MaeK and MaeR exert their function by activating the expression of L-malate catabolic genes (maeP and maeE) and the expression of their own genes upon the presence of L-malate in the medium. Structural and phylogenetic analyses show that L. casei MaeKR proteins belong to the citrate family of TCS, as well as the characterized DcuSR and CitAB TCS. We also solved the crystal structure of the REC domain of MaeR in its activated state as well as the structure of a mutant version defective in the phosphoacceptor Asp. Altogether, our analysis has revealed that MaeKR is a non-canonical TCS conserved in Lactobacillales and that the structure of MaeR acknowledges the α4β5α5-swapped dimers as a new class of dimerization for RRs.

In an attempt to determine the MaeR unphosphorylated monomeric conformation, we performed crystallization studies of a MaeRREC mutant form where D54 was replaced by an alanine (MaeRREC-D54A). MaeRREC-D54A crystallized in the same space group and similar size dimension than the wild-type MaeRREC. The determination of the structure of MaeRREC-D54A by molecular replacement revealed the presence of a swapped dimer into the unit cell identical to the one obtained for the wild type MaeRREC (RMSD is 0.52 Å for 242 residues). The crystals were obtained at high concentrations of sulfate (1.6 M) and it is well known that sulphates can mimic phosphate ions. No interactions with the conserved Asp9 were observed due to the absence of a magnesium ion in the active site. The residues Thr82 and Tyr101 forming the Y-T switch present the inward conformation as in the MaeRREC-BeF structure, confirming an activated state for MaeRREC-D54A. The fact that the non-phosphorylatable mutant also adopts a dimeric swapped conformation indicates that this conformation is not induced upon phosphorylation. On the contrary, it supports that the swapping by itself generates the conformation competent for phosphorylation where the active site displays an organization able to accept the phosphoryl group. This notion is further supported by the coordination of a sulphate ion in the absence of a phosphorylatable Asp in the MaeRREC-D54A crystals. EMSA assays showed that the D54A mutant had completely lost the capacity to bind the mae promoter.

>[2x]AATNILIVEDDPMVQFIHRNYLEKIGTFDTIYSSETIADAKKLLASRSIQLVLLAIRLKDGNGIDFLTDLRRTKQTVDVILITAANEVNIVNDALHLGVIDYLIKPFTLERFEKSIQRYRTK> GKNKQLRNDFKLVENILAKRLLILPQEEDYGFDIEEKNKAVVVKSVQRGSLAE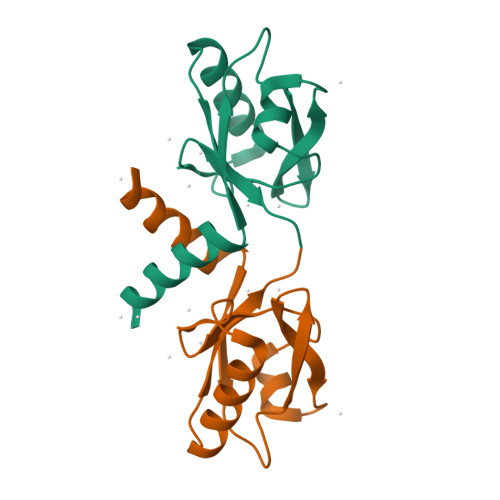VAGLQVGRKIYSINEDLVFLRPFSEVESILNQSFCSRRPLRLLVATKA> GLTEEQRMMIRELMDAQMKTFDTTFSHFKNFRLPGVLSSGCELPESLQAPSREEAAKWSQVRKDLCSLKVSLQLRGEDGSVWNYKPPADSGGKEIFSLLP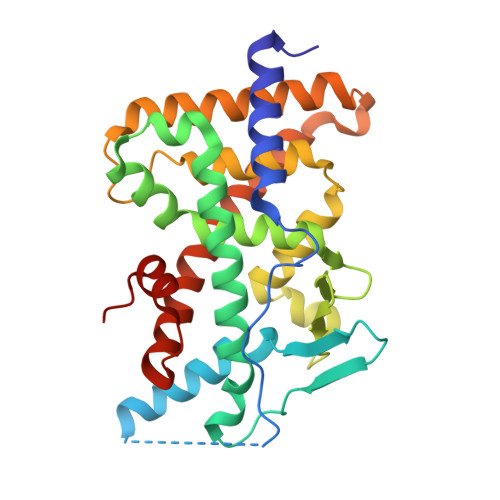HMADMSTYMFKGIISFAKVISYFRDLPIEDQISLLKGAAFELSQLRFNTVFNAETGTWECGRLSYCLEDTAGGFQQLLLEPMLKFHYMLKKLQLHEEEYVLMQAISLFSPDRPGVLQHRVVDQLQEQFAITLKSYIECNRPQPAHRFLFLKIMAMLTELRSINAQHTQRLLRIQDIHPFATPLMQELFGITGS> MLGLGGAATRQLTFQTSSPAHLTMPYVMPGDGEVVGVGEPVAIRFDENIADRGAAEKAIKITTNPPVEGAFYWLNNREVRWRPEHFWKPGTAVDVAVNTYGVDLGEGMFGEDNVQTHFTIGDEVIATADDNTKILTVRVNGEVVKSMPTSMGKDSTPTANGIYIVGSRYKHIIMDSSTYGVPVNSPNGYRTDVDWATQISYSGVFVHSAPWSVGAQGHTNTSHGCLNVSPSNAQWFYDHVKRGDIVEVVNTVGGTLPGIDGLGDWNIPWDQWRAGNAKALEHHHHHH

Among five paralogues of l,d-transpeptidase in Mtb, two functional l,d-­transpeptidases, LdtMt1 (Rv0116c; 251 amino acids) and LdtMt2 (Rv2518c; MT2594; 408 amino acids), have been shown to generate 3→3 cross-links connecting two meso-diaminopimelic acid (meso-DAP) residues at the third position of the stem peptides in vitro. Here, we report the crystal structure of an N-terminally truncated Mtb LdtMt2 (LdtMt2Δ130) that encompasses residues Leu131–Ala408. In this structure, the catalytic l,d-transpeptidase domain (residues Asp251–Val378) is preceded by a bacterial immunoglobulin-like (Ig-like) Big_5 domain (residues His150–Gly250) and followed by an extended C-­terminal tail (residues Asn379–Ala408) that interacts with both domains. Cys354, His336 and Ser337 form the catalytic triad in the active site of the l,d-transpeptidase domain.

We refined three models of LdtMt2Δ130: (i) the apo form, (ii) a mercury-derivatized ligand-free form and (iii) a meropenem-complexed form. The apo and mercury-derivatized crystals contained one monomer of LdtMt2Δ130 per asymmetric unit, whereas the crystals of the meropenem complex contained two monomers (chains A and B) in the asymmetric unit. In these models, the N-­terminal residues (Leu131–Ala149 in the apo form, Leu131–Thr145 in the mercury derivative and Leu131–Gln140 in the meropenem complex for both chains A and B) and C-terminal affinity tag (LEHHHHHH) are disordered. In the apo model, the internal region of the polypeptide chain (Ser305–Tyr318) is also disordered. The flexible nature of the active-site lid is further supported by the apo structure, in which much of the lid is disordered. Our crystals of apo LdtMt2Δ130 were obtained using a reservoir solution containing 50 mM calcium chloride, whereas the crystallization condition for the meropenem complex did not contain calcium ions. The r.m.s. deviation between the apo and mercury-derivative models is small (0.40 Å for 246 Cα-atom pairs), indicating that the mercury binding did not cause a large overall structural change. The largest surface area buried at the interface between two monomers of LdtMt2Δ130 within the crystals is 501 and 815 Å2 per monomer (4.5% and 6.6% of the monomer surface area) for the apo form and the mercury derivative (both in space group C2), respectively. Such monomer–monomer contacts can be regarded as crystallization artifacts. The weighted r.m.s. errors for the monomer (1×) and dimer (2×) fits are 7.93 × 10−3 and 4.88 × 10−2, respectively, demonstrating the superiority of the 1× model. The residual plots shown in Supplementary Fig. S3(b) also support our conclusion that apo LdtMt2Δ130 exists as monomers in solution.> MALEEIRPKEVYLDRKLLTLEDKELGSGNFGTVKKGYYQMKKVVKTVAVKILKNEANDPALKDELLAEANVMQQLDNPYIVRMIGICEAESWMLVMEMAELGPLNKYLQQNRHVTDKNIIELVHQVSMGMKYLEESNFVHRDLAARNVLLVTQHYAKISDFGLSKALRADENYYKAQTHGKWPVKWYAPECINYYKFSSKSDVWSFGVLMWEAFSYGQKPYRGMKGSEVTAMLEKGERMGCPAGCPREM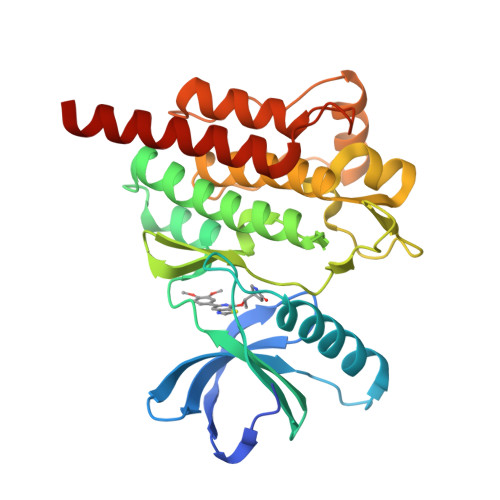YDLMNLCWTYDVENRPGFAAVELRLRNYYYDVVNHHHHHH>MGSSWSHPQFEKSSGLVPRGSHMLEQCPVTKIGPWGSSHEGTVQDITESPKRLESITLYHGWSVDSISFTYLDHAGEKHKAGPWGGPGGDPIMIEFGSSEFLKEVSGTFGPYEGSTVITSINFITNKQTYGPFGRQEGTPFSVPAQNNSSIVGFFGRSGKYINAVGVYVQPI[2x]

A protein involved in resistance against different pathogen groups, which is only present in monocot plants, is referred to as monocot chimeric jacalin (MCJ). As its name suggests, it is a fusion of two proteins, a jacalin-related lectin (JRL) and a dirigent protein (DIR) at the N-terminus. Therefore, the development of disease resistant plants is mandatory. It was shown that the rice (Oryza sativa) protein OsJAC1 enhances resistance against different bacterial and fungal plant pathogens in rice, barley, and wheat. Here, we report crystal structures for both individual domains and the complex of galactobiose with the DIR domain, which revealed a new carbohydrate binding motif for DIR proteins.

The JRL domain has a β-prism-I fold composed of three four-stranded antiparallel β-sheets. Two of these sheets are canonical Greek key motifs, whereas in the third case the very N- and C-terminal segments of the protein join to form the outer and inner pair of strands, respectively. The two dimeric assemblies of OsJAC1-JRL superpose with a root-mean-square (RMS) distance of 0.87 Å for Cα atoms and 1.24 Å for all non-hydrogen atoms (using residue range 160–306 in all subunits). The dimer itself features C2 symmetry with constituent chains being more similar in crystal form 1 of the OsJAC1-JRL domain (Cα RMS distance 0.58 Å) than in JRL-cf2 (Cα RMS distance 1.13 Å). As indicated by PISA analysis, the extensive interface involving both hydrophobic and polar interactions buries more than 800 Å2 of solvent-accessible surface area on either protomer and is classified as stable in solution. In contrast to all other mJRLs from plants, the two chains of the non-crystallographic dimer of OsJAC1-JRL are linked via a symmetric disulfide bond formed by a cysteine residue close to the N-terminus (Cys161). The possibility of disulfide bond formation for the JRL domain was already indicated in our previous work based on a shift in the thermal melting point upon oxidation. Overall, the intimate interaction between subunits suggests a physiologically relevant mode of dimerization; accordingly, the disulfide bond may not just represent an artefact of crystallization under non-reducing conditions but may actually occur in the full-length protein (see Discussion section). The increased hemagglutination activity of the OsJAC1-JRL domain under oxidizing conditions points to a crucial role of the intermolecular disulfide bond that is consistently observed in both crystal forms. Intriguingly, the hemagglutination activity of the separated JRL domain decreased up to 8-fold under reducing assay conditions (4 mM DTT). These observations suggest that, in contrast to full-length OsJAC1 and the DIR domain, the JRL domain relies on dimerization via the inter-subunit disulfide bond to achieve optimal hemagglutination activity.> MLITGDSIVSAEAVWDHVTMANR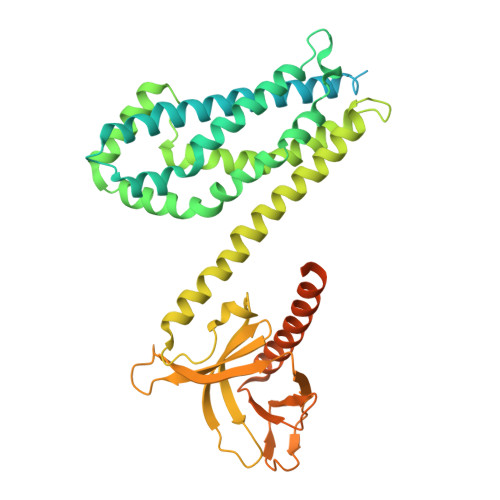GVAFKAGDVIKVLDASNKDWWWGQIDDEEGWFPASFVRLWVNQEDGVEEGPSDVQNGHLDPNSDCLCLGRPLQNRDQMRANVINEIMSTERHYIKHLKDICEGYLKQCRKRRDMFSDEQLKVIFGNIEDIYRFQMGFVRDLEKQYNNDDPHLSEIGPCFLEHQDGFWIYSEYCNNHLDACMELSKLMKDSRYQHFFEACRLLQQMIDIAIDGFLLTPVQKICKYPLQLAELLKYTAQDHSDYRYVAAALAVMRNVTQQINERKRRLENIDKIAQWQASVLDWEGDDILDRSSELIYTGEMAWIYQPYGRNQQRVFFLFDHQMVLCKKDLIRRDILYYKGRIDMDKYEVIDIEDGRDDDFNVSMKNAFKLHNKETEEVHLFFAKKLEEKIRWLRAFREERKMVQEDEKIGFEISENQKRQAAMTVRKASKQKGRVGEEENQSLELKRACEVLQRLWSPGKKSC>ERLSTLIHQRMQEAKVPALSVSVTIKGVRQRFVYGVADVASQKANTLDTVYELGSMSKAFTGLVVQILIQEGRLRQGDDIITYLPEMRLNYQGKPASLTVADFLYHTSGLPFSTLARLENPMPGSAVAQQLRNENLLFAPGAKFSYASANYDVLGAVIENVTGKTFTEVIAERLTQPLGMSATVAVKGDEIIVNKASGYKLGFGKPVLFHAPLARNHVPAAYIHSTLPDMEIWIDAWLHRKALPATLREAMSNSWRGNSDVPLAADNRILY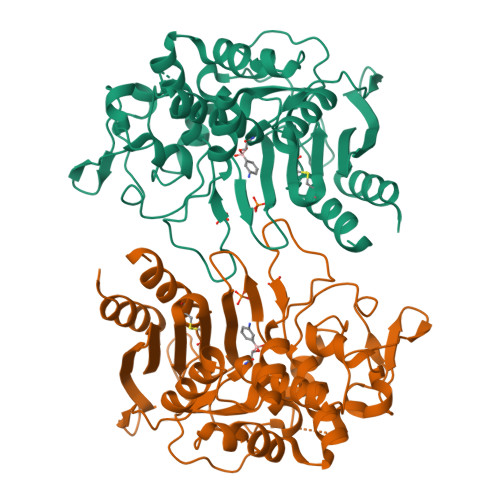ASGWFIDQNQGPYISHGGQNPNFSSCIALRPDQQIGIVALANMNSNLILQLCADIDNYLRIGKY[3x]(2R)-2,4-dihydroxy-N-[2-(7-hydroxy-1H-benzimidazol-2-yl)ethyl]-3,3-dimethylbutanamide | C15 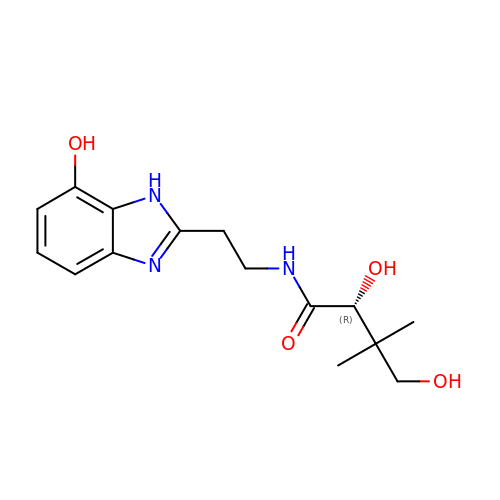H21 N3 O4 | SKIDJNQZVCDYIE-ZDUSSCGKSA-N>MRGSHHHHHHGSSTQRHVRIGIIGGGPAGLTAGIYASRANLKTCVFVGIEHTSQMFTTTDVENFPSHTAIKGPALMEAIQNQAEHCGAELLYEDVHSIDVSSRPFKIVHGYENETTLADALIIATGATARRLDCKGEKEYWQKGVSACAVCDSAMATGKEVVVVGGGDVACEEATYLTKIATKVYMVLRRDKFRASAAMV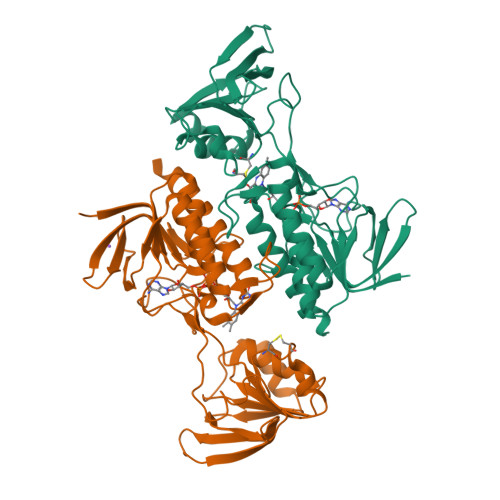KKVMNEKLIEIIYDSAIDEIKGDGKCVTSVSIKNLKDGKTRTLNAGALYWAVGHDPQTSFLKKGQLEQDEAGYILLKDHPTQRTSVDGVFAAGDCCDHLYRQAVVAAGSGSKAALDAERWLAMQE[2x]>MAMANNSSVANKVCLIVIDGWGVSEDPYGNAILNAQTPVMDKLCSGNWAQIEAHGLHVGLPEGLMGNSEVGHLNIGAGRVIYQDIVRINLAVKNNKFVTNESLVDACDRAKNGNGRLHLAGLVSDGGVHSHIDHMFALVKAIKELGVPELYLHFYGDGRDTSPNSGVGFLEQTLEFLEKTTGYGKLATVVGRYYAMDRDNRWERINVAYEAMIGGVGETSDEAGVVEVVRKRYAADETDEFLKPIILQGEKGRVQNDDTIIFFDYRADRMREISAAMGMDRYKDCNSKLAHPSNLQVYGMTQYKAEFPFKSLFPPASNKNVLAEWLAEQKVSQFHCAETEKYAHVTFFFNGGLEKQFEGEERCLVPSPKVATYDLQPEMSAAGVADKMIEQLEAGTHPFIMCNFAPPDMVGHTGVYEAAVKACEATDIAIGRIYEATQKHGYSLMVTADHGNAEKMKAPDGGKHTAHTCYRVPLTLSHPGFKFVDPADRHPALCDVAPTVLAIMGLPQPAEMTGVSIVQKIKLAAALEHHHHHHHHHH[2x];>XYDYPGDFCYLYGTCX[2x]

In all vertebrates, cofactor-dependent phosphoglycerate mutase (dPGM) is a 2, 3-bisphophoglycerate cofactor–utilizing homodimer consisting of 23-kDa subunits, while the parasitic enzyme is a 56-kDa monomer cofactor-independent enzyme consisting of a phosphatase domain connected by a flexible hinge to the phosphotransferase domain. In dPGM, an active site phosphohistidine (H10) equilibrates the phosphate between the 2 and 3 positions of glyceric acid, while in cofactor-independent phosphoglycerate mutase (iPGM), a transition metal ion–activated serine (S86) mediates the phosphate transfer. We previously discovered ipglycermide, a potent inhibitor of iPGM, from a large combinatorial cyclic peptide library. Our results show that the high-affinity binding of ipglycermide to iPGMs freezes these structurally dynamic enzymes into an inactive, stable complex.

To gain structural insight into the molecular interactions of the C-terminus of ipglycermides with iPGM, we established co-crystal structures using analogs, Ce-2 Tyr7Phe and Ce-1 Cys14NHOH (Ce-1 NHOH), respectively, retaining Cys14 or replacing it with NHOH, an oxidation-insensitive and solid-phase peptide synthesis (SPPS)-accessible metal-ion–coordinating ligand. Using our established crystallization conditions, supplemented with 2-mM tris(2-carboxyethyl)phosphine for Ce-2 Tyr7Phe–containing complexes, we were able to obtain crystals diffracting to 2.1 Å and 1.80 Å for Ce-2 Tyr7Phe and Ce-1 NHOH, respectively, bound to C. elegans iPGM. Comparable hydrogen-bond interactions that were observed in iPGM⋅Ce-1 NHOH are present in the iPGM⋅Ce-2 Tyr7Phe structure. However, residues 12 to 14 of Ce-2 Tyr7Phe and Ce-1 NHOH display nonoverlapping conformations resulting from differences in Zn2+ coordination. In the iPGM–Ce-2 Tyr7Phe complex, the Cys14-NH2 residue forms a monodentate interaction with the Zn2+ through the S atom (2.28 Å) as suggested by prior modeling using the C. elegans iPGM–Ce-2d complex. In addition, the Cys14-terminal amide NH2 group forms an intramolecular hydrogen bond with Tyr11, possibly serving to brace and position the Cys14 thiolate. From this binding orientation, it can be envisioned how the nucleic acid attached to the C terminus of the original RNA-encoded ligand could be accommodated in the complex. The main change in the common sequence is observed for residue Thr13 that is displaced from the Zn2+ in iPGM–Ce-2 Tyr7Phe to accommodate the binding of Cys14. Notably, the sulfur atom of Cys14 is positioned in a nearly identical region as the Thr13/hydroxamate carbonyl in the iPGM⋅Ce-1 NHOH structure. Despite these conformational displacements, the Thr13 side-chain hydroxyl adopts a similar spatial position in both structures, thereby maintaining the hydrogen-bond interaction with the phosphatase domain E87 γ-carboxylate.>DLIDRLQNNQRKDRRLQFVRTHQEAFDVKPTFPLPLFEEAILEIEGSCSVESSCQVEGDRLQGGRYEVCNNQGTTWPESLTHAFKLLDKIDSQLGVRINRDSFDRFAAAHVNSRKIINNTIGVHLGSKLEDSSVMLYIHIKPEEDTEELARTALVLDGGRYSDELTRVLLRDTMVIGFELFFDGRSRVDLGPCAPGKSGTLKMKGKHLEQYTQKNLSRKVNSIFREGYLFGAFFSKTRVEPILFFYHSIIKDLPKYFTFNSLGDKIYNFCQS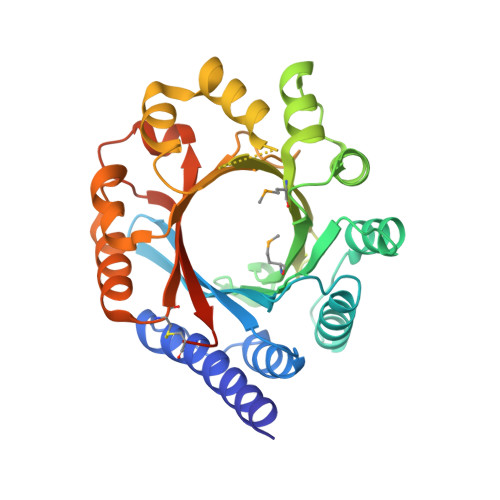QGCITDVAIAVTETELEKSRLENFCFYYDQWDECKPSSDYDTERHLHRS[2x]>[2x]MQSDTQEVNDITTLATLHYNGSTP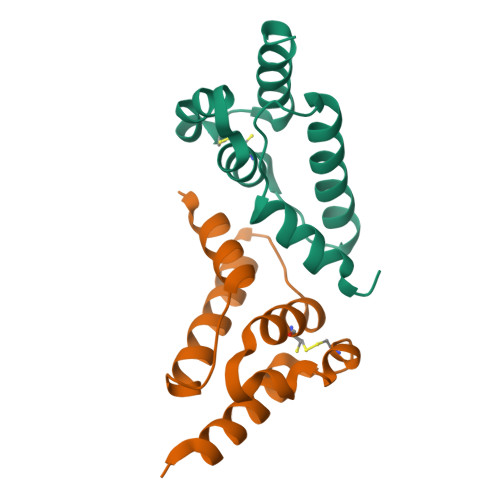ADAFEAEVTNILDRLNNNGIPINNKVACQFIMRGLSGEYKSLRYARHRCIHMTVADLFSDIHSMYEEQQPLEH>AFVVTDNCIKCKCTDCVEVCPVDCFYEGPNFLVIHPDECIDCALCEPECPAQAIFSEDEVPEDMQEFIQLNAELAEVWPNITEKKDPLPDAEDWDGVKGKLQHL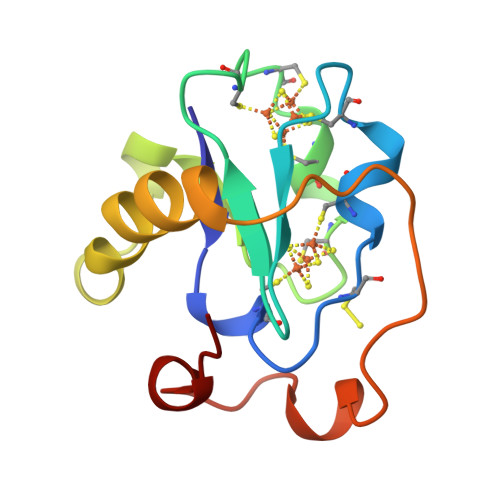ER[2x]> MHHHHHHHHLEVLFQGPTSDIQTYTSINKYEVPPAYSRLPLTSGRFGTDNFDFTPFNNTEYSGLDPDVDNHYTNAIIQLYRFIPEMFNFVVGCLKDENFETTLLTDLGYLFDMMERSHGKICSSSNFQASLKSLTDKRQLENGEPQEHLEEYLESLCIRESIEDFNSSESIKRNMPQKFNRFLLSQLIKEEAQTVNHNITLNQCFGLETEIRTECSCDHYDTTVKLLPSLSISGINKTVIKQLNKKSNGQNILPYIEYAMKNVTQKNSICPTCGKTETITQECTVKNLPSVLSLELSLLDTEFSNIRSSKNWLTSEFYGSIIKNKAVLRSTASELKGTSHIFKYELNGYVAKITDNNNETRLVTYVKKYNPKENCFKWLMFNDYLVVEITEEEALKMTYPWKTPEIIIYCDAEELRKPFFSVDTYSINYDILFRDYFANGIRDTARREYKLLTHDEAPKS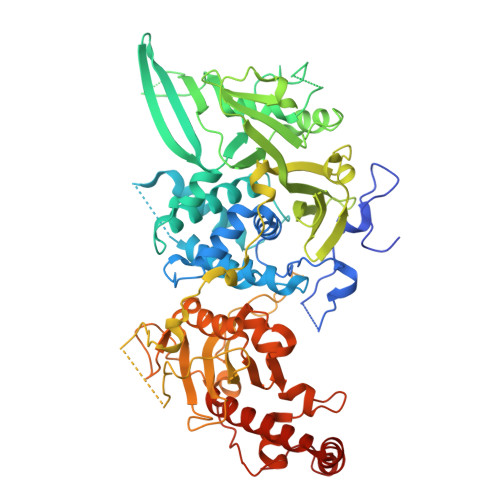GTLVAIDAAFVSLQSELCEIDHQGIRSIIRPKRTALARISIIRGEEGELYGVPFVDDYVVNTNHIEDYLTRYSGILPGDLDPEKSTKRLVRRNVVYRKVWLLMQLGCVFVGHGLNNDFKHININVPRNQIRDTAIYFLQGKRYLSLRYLAYVLLGMNIQEGNHDSIEDAHTALILYKKYLHLKEKAIFEKVLNSVYEEGRAHNFKVPETSKG(1Z,3E)-5-carboxy-3-methyl-5-oxo-1-phenylpenta-1,3-dien-1-olate 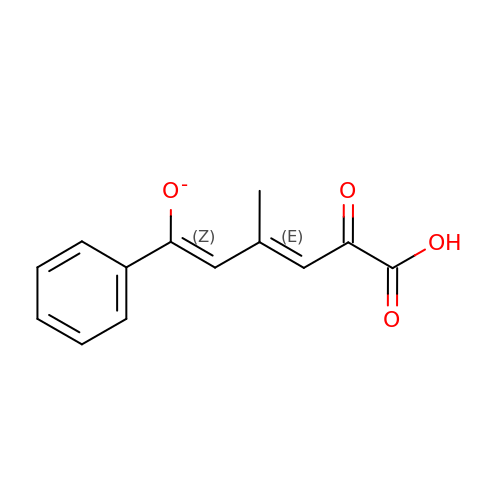| C13 H11 O4 | JCSKQBIZFFCCKU-UVTPKQPNSA-M>[2x]MRGSHHHHHHTDPHAAAAGVIPVGDSRVYGAVFDKGRKLTVNQWQAVLSMDAYPENGTTNYQEVGPWRYCEVDYEAAQGISDYRGDTFGPVGVTTVGDFPDYFKKAFAPYVLGKSNATNADMLAWGVQVTGVTAGNFQADDTALDPYPSKSRSDKNKRAALTKICGALQSAFDTQQDKYVMSHYAHIDQDKLVPVLNALKGIGFTAFDRYNLVGLAFQVQVNT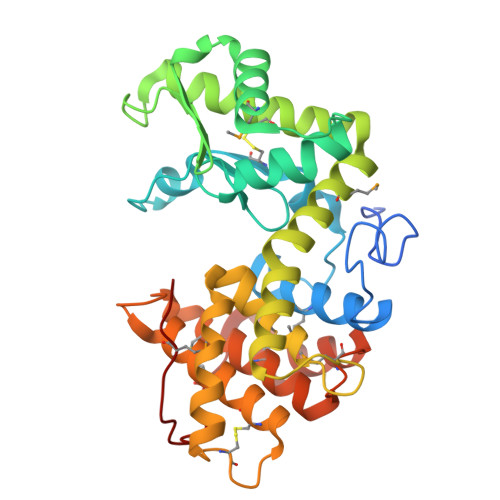GSIGSISAFSSVKSAGNCGSLSAETCFATYLTDQYIRWLKSSSLGDDPDNCWRASMALDIYKKDPTMGSVSVVNQVINASYPGNSGKCPTSGIKWSKNMSWQ>AMEQCGRQAGGALCPGGLCCSQYGWCA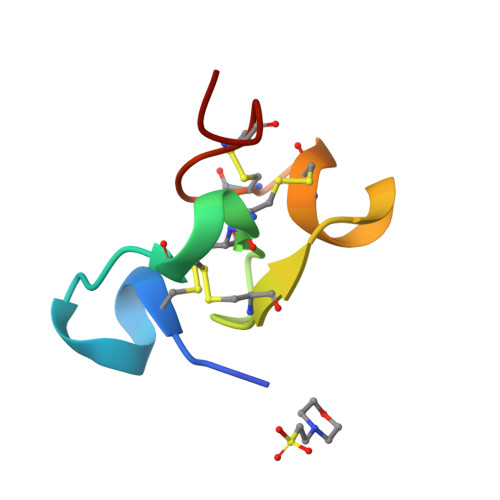NTPEYCGSGCQSQCDGGV[2x]>XEVKQLEAEVEELESELWHLENEVARLEKENAECEA[3x];>[3x]XKVKQLKAKVEELKSKLWHLKNK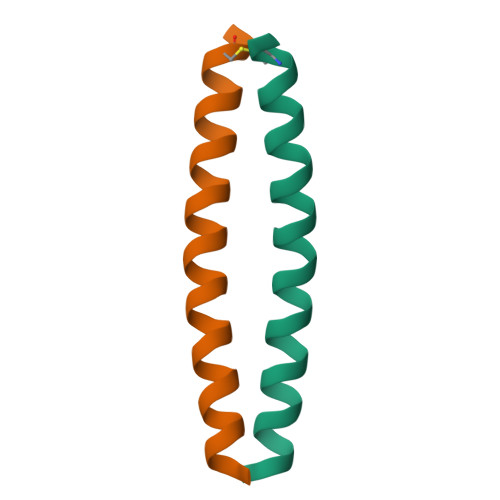VARLKKKNAECKA> GPLSLSVDAFKILEDPKWEFPRKNLVLGKTLGEGEFGKVVKATAFHLKGRAGYTTVAVKMLKENASPSELRDLLSEFNVLKQVNHP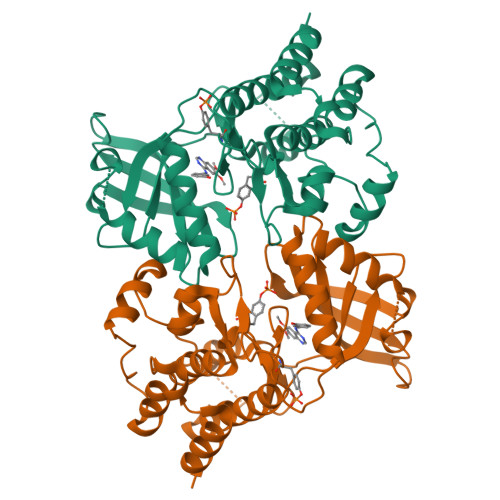HVIKLYGACSQDGPLLLIVEYAKYGSLRGFLRESRKVGPGYPDERALTMGDLISFAWQISQGMQYLAEMKLVHRDLAARNILVAEGRKMKISDFGLSRDVYEEDSYVKRSQGRIPVKWMAIESLFDHIYTTQSDVWSFGVLLWEIVTLGGNPYPGIPPERLFNLLKTGHRMERPDNCSEEMYRLMLQCWKQEPDKRPVFADISKDLEKMMVKR>MGNNLMQTDLSVWGMYQHADIVVKCVMIGLILASVVTWAIFFSKSVEFFNQKRRLKREQQLLAEARSLNQANDIAADFGSKSLSLHLLNEAQNELELSEGSDDNEGIKERTSFRLERRVAAVGRQMGRGNGYLATIGAISPFVGLFGTVWGIMNSFIGIAQTQTTNLAVVAPGIAEA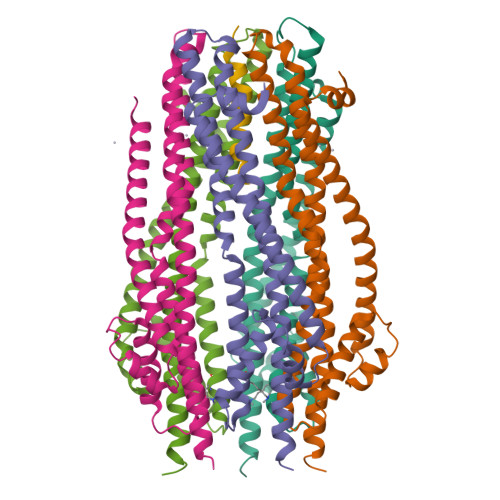LLATAIGLVAAIPAVVIYNVFARQIGGFKAMLGDVAAQVLLLQSRDLDLEASAAAHPVRVAQKLRAG[10x];>[2x]MAMHLNENLDDNGEMHDINVTPFIDVMLVLLIIFMVAAPLATVDVKVNLGGGENLYFQ> GPLGSMTTDEGAKNNEESPTATVAEQGEDITSKKDRGVLKIVKRVGNGEETPMIGDKVYVHYKGKLSNGKKFDSSHDRNEPFVFSLGKGQVIKAWDIGVATMKKGEICHLLCKPEYAYGSAGSLPKIPSNATLFFEIELLDFKGEDLFEDGGIIRRTKRKGEGYSNPNEGATVEIHLEGRCGGRMFDCRDVAF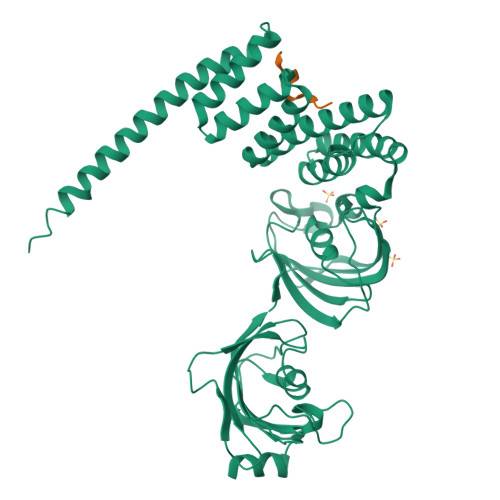TVGEGEDHDIPIGIDKALEKMQREEQCILYLGPRYGFGEAGKPKFGIEPNAELIYEVTLKSFEKAKESWEMDTKEKLEQAAIVKEKGTVYFKGGKYMQAVIQYGKIVSWLEMEYGLSEKESKASESFLLAAFLNLAMCYLKLREYTKAVECCDKALGLDSANEKGLYRRGEAQLLMNEFESAKGDFEKVLEVNPQNKAARLQISMCQKKAKEHNERDRRIYANMFKKFAEQDAKEEANKAMGKKTSEGVTNEKGTDSQAMEEEKPEGHV;> HHHHHHDDTSRMEEVD>SNATFLELVEVPCNSVHVQGVMTPNQMVKVTGAGWDNGVLEFYVTRPTKTGGDTSRSHLASIMCYSKDIDGVPSDKAGKCFLKRFSGEDSSEIDEKEVSLPIKSHNDAFMFVCSSNDGSALQCDVFALDNTNSNDGWKVNTVDLGVSVSPDLAFGLTADGVKVKKLYASSGLTAINDDPSLGCKA[3x]

Microneme protein 2 (MIC2) and MIC2-associated protein (M2AP) play crucial roles in the gliding motility and host cell invasion of Toxoplasma gondii. Complex formation between MIC2 and M2AP is required for maturation and transport from the microneme to the parasite surface. MIC2 contains a von Willebrand factor type A (VWA) domain and six tandem thrombospondin type 1 repeat (TSR) domains in its ectodomain. In this study, we report crystal structures of M2AP alone and in complex with TSR6.

The optimized crystals of M2AP β-domain alone (we referred as M2AP hereinafter) and its complex with TSR6 diffracted to high resolution (1.8–2 Å). However, structure of M2AP alone could not be solved using molecular replacement with the previous NMR model. Thus, experimental phasing with a selenium derivative was used instead. The crystal and previous NMR structure showed that M2AP has a galectin-like fold comprising 13 antiparallel strands. These strands form two β-sheets that make up two opposite faces, with one face being more hydrophobic than the other. The binding on the M2AP side is quite rigid, as only slight variations were identified when comparing the complex structure with the M2AP-only structure. Notable differences include the Trp-180 bearing loop region that moves slightly toward the TSR6, consistent with previous literature identifying Trp-180 and its nearby hydrophobic patch as the key region for binding with MIC213.> KVAYLTFDDGPGKYTAELLNTLKQHDAKATFFLIGANVKEFPDLVKRENAEGHYVGMHSMTHNFAKLYKNGEYVNEMKEDQGLIANIIGKSPKLTRPPYGSMPGLNEGLRNKVVEGGFKVWDWTIDSLDWRYNKMPVDAAAAQIAQNVLTNATKPQEVILMHDIHPQSVAAVPAILKGLKEKGYEFEAYHEESHFPVNFWHDNRM;>MEKALKIKQIVVVLIAIAAVAIGYYMFQSITSPAKAVAKQENVVQLASEQPKVEMNKTA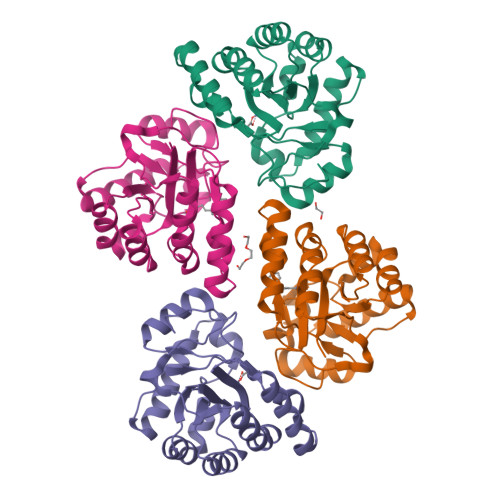PSRFNGKERKVAYLTFDDGPGKYTAELLNTLKQHDAKATFFLIGANVKEFPDLVKRENAEGHYVGMHSMTHNFAKLYKNGEYVNEMKEDQGLIANIIGKSPKLTRPPYGSMPGLNEGLRNKVVEGGFKVWDWTIDSLDWRYNKMPVDAAAAQIAQNVLTNATKPQEVILMHDIHPQSVAAVPAILKGLKEKGYEFEAYHEESHFPVNFWHDNRM[3x]>[3x]ATND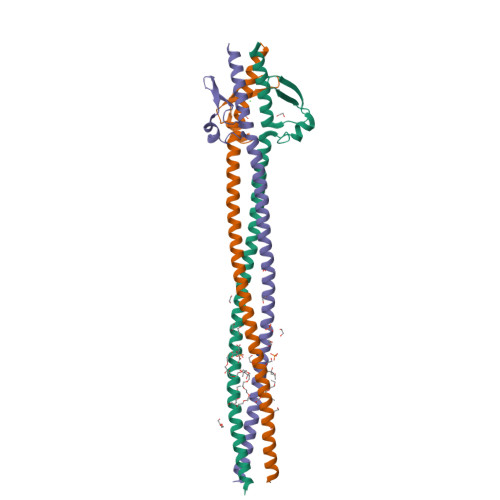DDVKKAATVAIAAAYNNGQEINGFKAGETIYDIDEDGTITKKDATAADVEADDFKGLGLKKVVTNLTKTVNENKQNVDAKVKAAESEIEKLTTKLADTDAALADTDAALDATTNALNKLGENITTFAEETKTNIVKIDEKLEAASKHHHHHH> TGEENCNVNNGGCAQKCQMIRGAVQCTCHTGYRLTEDGRTCQDVNECAEEGYCSQGCTNSEGAFQCWCEAGYELRPDRRSCKALGPEPVLLFANRIDIRQVLPHRSEYTLLLNNLENAIALDFHHRRELVFWSDVTLDRILRANLNGSNVEEVVSTGLESPGGLAVDWVHDKLYWTDSGTSRIEVANLDGAHRKVLLWQSLEKPRAIALHPMEGTIYWTDWGNTPRIEASSMDGSGRRIIADTHLFWPNGLTIDYAGRRMYWVDAKHHVIERANLDGSHRKAVISQGLPHPFAITVFEDSLYWTDWHTKSINSANKFTGKNQEIIRNKLHFPMDIHTLHPQRQPAGKNRCGDNNGGC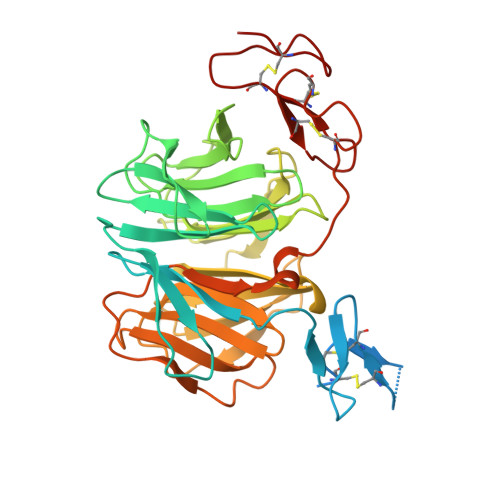THLCLPSGQNYTCACPTGFRKINSHACAQ5'-O-[(3-Indolyl)-1-Ethyl]Carbamoyl 2-aminoethenoadenosine 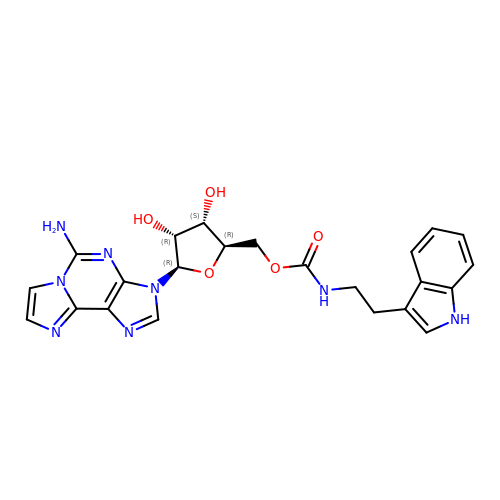| C23 H24 N8 O5 | PHVKAGZMQNJNJY-QTQZEZTPSA-N>[2x]MTIKWIDWVKQIQSIAQAGLTYSKDVYDIERFQQLRDISISMM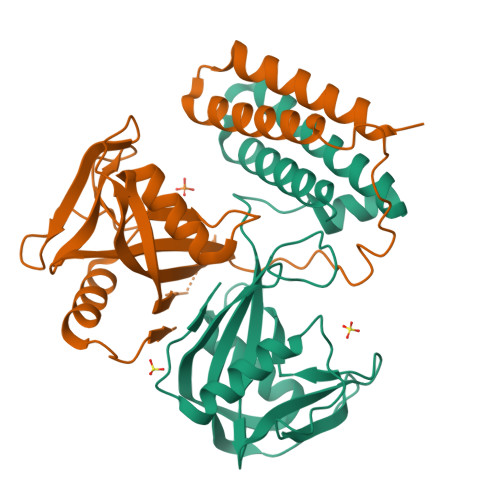SHYTKTDWEVVEKLFASETGYQTPKVDIRAVVFQNEKLLFVKEKSDGKWALPGGWADVGYTPTEVAAKEVFEETGYEVDHFKLLAIFDKEKHQPSPSATHVYKIFIGCEIIGGEKKTSIETEEVEFFGENELPNLSIARNTEDQIKEMFAYMKDPQKEKLID> MTTLRAFTCDDLFRFNNINLDPLTETYGIPFYLQYLAHWPEYFIVAEAPGGELMGYIMGKAEGSVAREEWHGHVTALSVAPEFRRLGLAAKLMELLEEISERKGGFFVDLFVRVSNQVAVNMYKQLGYSVYRTVIEYYSASNGEPDEDAYDMRKALSRDTEKKSIIPLPHPVRPEDIE;> XXXXXXXXXXXXXXXXXXXXXXXXXXXXHCAKVLKAIGLQRTGKQEEAFTLAQEVAALEPTDDNSLQALTILYREMHRPELVTKLYEAAVKKVPNSEEYHSHLFMAYARVGEYKKMQQAGMALYKIVPKNPYYFWSVMSLIMQSISAQDENLSKTMFLPLAERMVEKMVKEDKIEAEAEVELYYMILERLGKYQEALDVIRGKLGEKLTSEIQSRENKCMAMYKKLSRWPECNALSRRLLLKNSDDWQFYLTYFDSVFRLIEEAWSPPAEGEHSLEGEVHYSAEKAVKFIEDRITEESKSSRHLRGPHLAKLELIRRLRSQGCNDEYKLGDPEELMFQYFKKFGDKPCCFTDLKVFVDLLPATQCTKFINQLLGVVPLSTPTEDKLALPADIRALQQHLCVVQLTRLLGLYHTMDKNQKLSVVRELMLRYQHGLEFGKT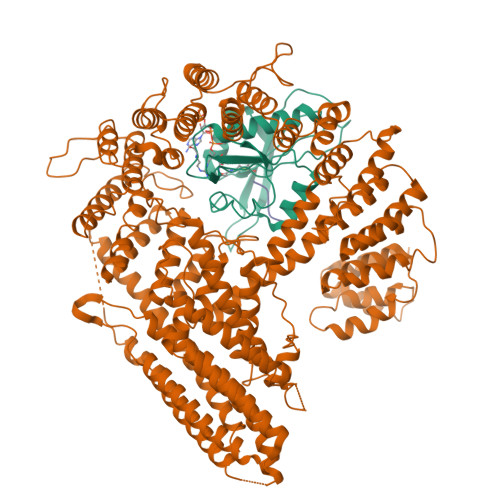CLKTELQFSDYYCLLAVHALIDVWRETGDETTVWQALTLLEEGLTHSPSNAQFKLLLVRIYCMLGAFEPVVDLYSSLDAKHIQHDTIGYLLTRYAESLGQYAAASQSCNFALRFFHSNQKDTSEYIIQAYKYGAFEKIPEFIAFRNRLNNSLHFAQVRTERMLLDLLLEANISTSLAESIKSMNLRPEEDDIPWEDLRDNRDLNVFFSWDPKDRDVSEEHKKLSLEEETLWLRIRSLTLRLISGLPSLNHPVEPKNSEKTAENGVSSRIDILRLLLQQLEATLETGKRFIEKDIQYPFLGPVPTRMGGFFNSGCSQCQISSFYLVNDIYELDTSGLEDTMEIQERIENSFKSLLDQLKDVFSKCKGDLLEVKDGNLKTHPTLLENLVFFVETISVILWVSSYCESVLRPYKLNLQKKKKKKKETSIIMPPVFTSFQDYVTGLQTLISNVVDHIKGLETHLIALKLEELILEDTSLSPEERKFSKTVQGKVQSSYLHSLLEMGELLKKRLETTKKLKI;> XMDVFM> GPLGSEKIEKDNAFAFDLLQTTRKHVTEANVFISPLSVSMALNMTLNGAAGVTADEMKTALRETGYTMEDINEYSHSLREALLKVDPSTTIGMANSIWYKQGELVKEPFILANRTHYDAEVKAVDFSSPATLPAINGWCAQKTNDKITKILDYIPGNAFMYLINAVYFKGIWVTQFKKSDTKRAPFRKA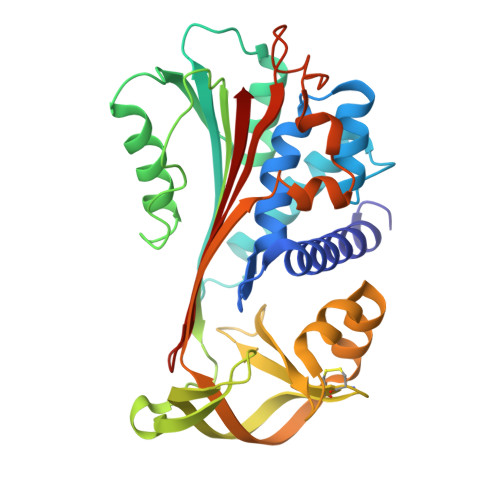DGTTQEVNMMAQKSTFGYTTDECCQYLEMDYGNKAFSMIVMLPNEGQTTRDVIEQLDNKHWSMIIKGIRPTQVSLRMPRFKTECKYGLEKKILPEMGMNVPFTETADFPGITDAAIFISRVIHKTFVQVDEEGTEAAAVTAVEMK> MKKANEALTRNRELTTVLVKNLPKSYNQNKVYKYFKHCGPIIHVDVADSLKKNFRFARIEFARYDGALAAITKTHKVVGQNEIIVSHLTECTLWMTNFPPSYTQRNIRDLLQDINVVALSIRLPSLRFNTSRRFAYIDVTSKEDARYCVEKLNGLKIEGYTLVTKVSNPLEKSKRTDSATLEGREIMIRNLSTELLDENLLRESFEGFGSIEKINIPAGQKEHSFNNCCAFMVFENKDSAERALQMNRSLLGNREISVSLADKKPFLERNEVKRLLASRNSKELETLICLFPLSDKVSPSLICQFLQEEIHINEKDIRKILLVSDFNGAIIIFRDSKFAAKMLMILNGSQFQGKVIRSGTINDMKRYYNNQQNHSMKHVKPSCINMMEKGPNL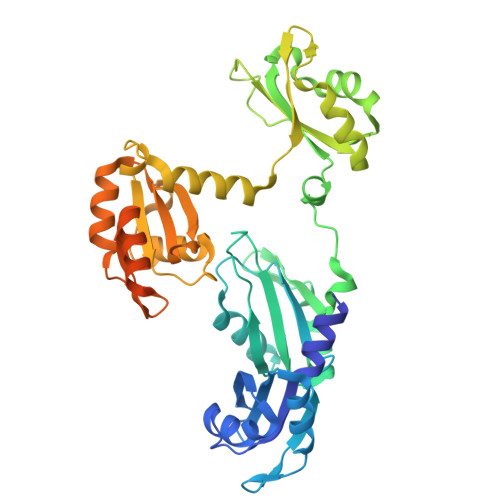QVKKKIPDKQEQMSNDDFRKMFLGEHHHHHH>[2x]MLVEGSELQSGAQQPRTEAPQHGELQYLRQVEHIMRCGFKKEDRTGTGTLSVFGMQARYSLRDEFPLLTTKRVFWKGVLEELLWFIKGSTNAKELSSKGVRIWDANGSRDFLDSLGFSARQEGDLGPVYGFQWRHFGADYKDMDSDYSGQGVDQLQKVIDTIKTNPDDRRIIMCAWNPKDLPLMALPPCHALCQFYVVNGELSCQLYQ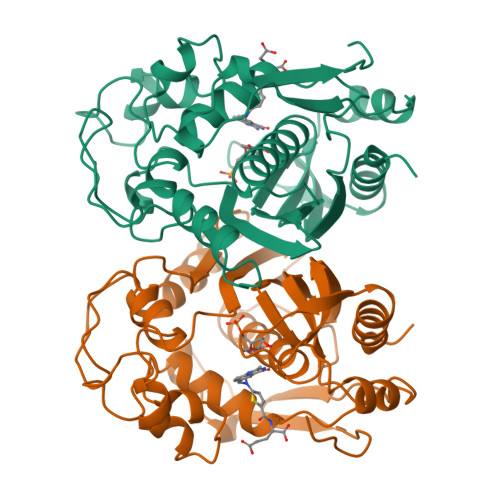RSGDMGLGVPFNIASYALLTYMIAHITGLQPGDFVHTLGDAHIYLNHIEPLKIQLQREPRPFPKLRILRKVETIDDFKVEDFQIEGYNPHPTIKMEMAV> GDSLSIHQLAAQGELDQLKEHLRKGDNLVNKPDERGFTPLIWASAFGEIETVRFLLEWGADPHILAKERESALSLASTGGYTDIVGLLLERDVDINIYDWNGGTPLLYAVRGNHVKCVEA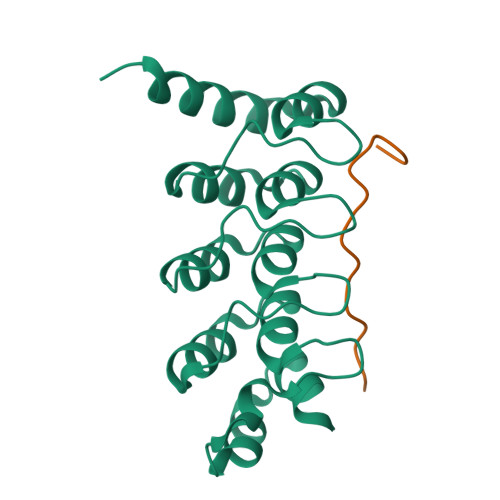LLARGADLTTEADSGYTPMDLAVALGYRKVQQVIENHILKLFQSNLVPADPE;> KTLVSMPPLPGLDLKGS> GSMAQNAEKDTLIVASKVKAYIKSKGFMTSGDAVDGLNEKLYALIDDALKRTESNKRTTVRP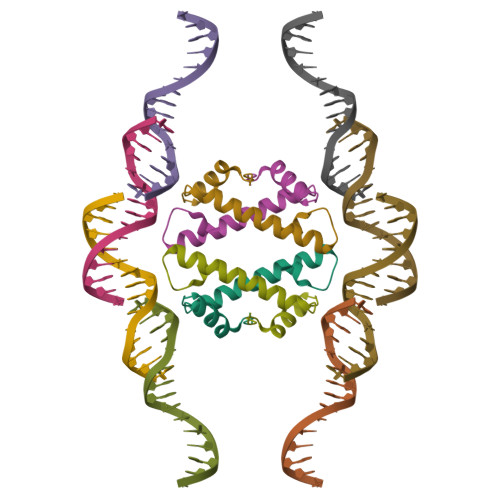TDF>MELIEVQEGKAKILIPKAESIYDSPVFYNPRMALNRDIVVVLLNILNPKIVLDALSATGIRGIRFALETPAEEVWLNDISEDAYELMKRNVMLNFDGELRESKGRAILKGEKTIVINHDDANRLMAERHRYFHFIDLDPFGSPMEFLDTALRSAKRRGILGVTATDGAPLCGAHPRACLRKYLAVPLRGELCHEVGTRILVGVIARYAAKYDLGIDVILAYYKDHYFRAFVKLKDGARKGDETLEKLGYIYFDDKTGKFELEQGFLPTRPNAYGPVWLGPLKDEKIVSKMVKEAESLSLARKKQALKLLKMIDQELDIPLFYDTHAIGRRLKI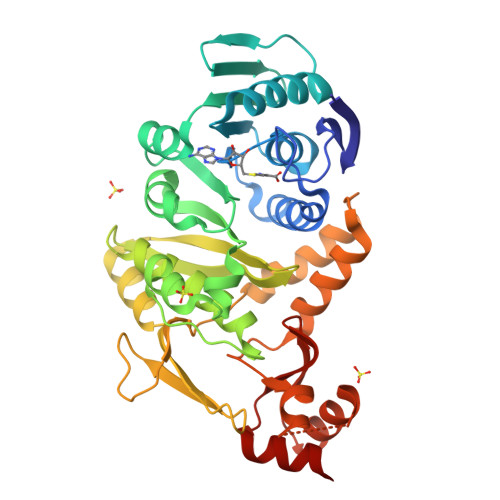ETKKVEEIISALREQGYEATRTHFSPTGIKTSAPYEVFIETIKRI[2x]> MKKEKIDLFYGALLADIGKVIQRATGERKKHALVGADWFDEIADNQVISDQIRYHMANYQSDKLGNDHLAYITYIADNIASGVDRRQSNEESDEDTSAKIWDTYTNQADIFNVFGAQTDKRYFKPTVLNLKSKPNFASATYEPFSKGDYAAIATRIKNELAEFEFNQVQIDSLLNLFEATLSFVPSSTNTKEIADISLADHSRLTAAFALAIYDYLEDKGRHNYKEDLFTKVSAFYEEEAFLLASFDLSGIQDFIYNINIATNGAAKQLKARSLYLDFMSEYIADSLLDKLGLNRANMLYVGGGHAYFVLANTEKTVETLVQFEKDFNQFLLANFQTRLYVAFGWGSFAAKDIMSELNSPESYRQVYQKASRMISKKKISRYDYQTLMLLNRGGKSSERECEICHSVENLVSYHDQKVCDICRGLYQFSKEIAHDHFIITENEGLPIGPNACLKGVAFEKLSQEAFSRVYVKNDYKAGTVKATHVFVGDYQCDEIYNYAALSKNENGLGIKRLAVVRLDVDDLGAAFMAGFSQQGNGQYSTLSRSATFSRSMSLFFKVYINQFASDKKLSIIYAGGDDVFAIGSWQDIIAFTVELRENFIKWTNGKLTLSAGIGLFADKTPISLMAHQTGELEEAAKGNEKDSISLFSSDYTFKFDRFITNVYDDKLEQIRYFFNHQDERGKNFIYKLIELLRNHDRMNMARLAYYLTRLEELTRETDRDKFKTFKNLFYSWYTNKNDKDRKEAELALLLYIYEIRKD;> MTYKLYIMTFQNAHFGSGTLDSSKLTFSADRIFSALVLEALKMGKLDAFLAEANQDKFTLTDAFPFQFGPFLPKPIGYPKHDQIDQSVDVKEVRRQAKLSKKLQFLALENVDDYLNGELFENEEHAVIDTVTKNQPHKDDNLYQVATTRFSNDTSLYVIANESDLLNELMSSLQYSGLGGKRSSGFGRFELDIQNIPLELSDRLTKNHSDKVMSLTTALPVDADLEEAMEDGHYLLTKSSGFAFSHATNENYRKQDLYKFASGSTFSKTFEGQIVDVRPL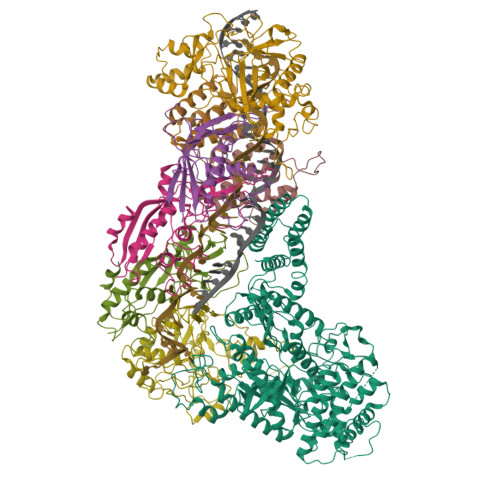DFPHAVLNYAKPLFFKLEV;>MTILTDENYVDIAEKAILKLERNTRNRKNPDAFFLTTSKLRNLLSLTSTLFDESKVKEYDALLDRIAYLRVQFVYQAGREIAVKDLIEKAQILEALKEIKDRETLQRFCRYMEALVAYFKFYGGKD[2x];>MTFAKIKFSAQIRLETGLHIGGSDAFAAIGAINSPVIKDPITNLPIIPGSSLKGKMRTLLAKVYNEKVAEKPSDDSDILSRLFGNSKDKRFKMGRLIFRDAFLSNADELDSLGVRSYTEVKFENTIDRITAEANPRQIERAIRNSTFDFELIYEITDENENQVEEDFKVIRDGLKLLELDYLGGSGSRGYGKVAFENLKATTVFGNYDVKTLNELLTAEV[3x];> MKNDYRTFKLSLLTLAPIHIGNGEKYTSREFIYENKKFYFPDMGKFYNKMVEKRLAEKFEAFLIQTRPNARNNRLISFLNDNRIAERSFGGYSISETGLESDKNPNSAGAINEVNKFIRDAFGNPYIPGSSLKGAIRTILMNTTPKWNNENAVNDFGRFPKENKNLIPWGPKKGKEYDDLFNAIRVSDSKPFDNKSLILVQKWDYSAKTNKAKPLPLYRESISPLTKIEFEITTTTDEAGRLIEELGKRAQAFYKDYKAFFLSEFPDDKIQANLQYPIYLGAGSGAWTKTLFKQADGILQRRYSRMKTKMVKKGVLKLTKAPLKTVKIPSGNHSLVKNHESFYEMGKANFMIKEIDK1,3-benzothiazol-2-amine | C7 H6 N2 S | 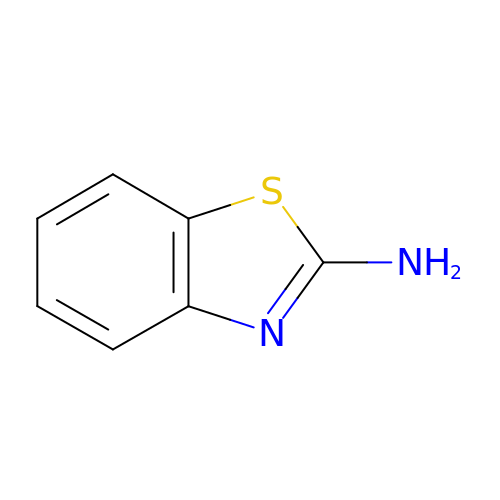UHGULLIUJBCTEF-UHFFFAOYSA-N(4-phenoxyphenyl)methanol | C13 H12 O2 | 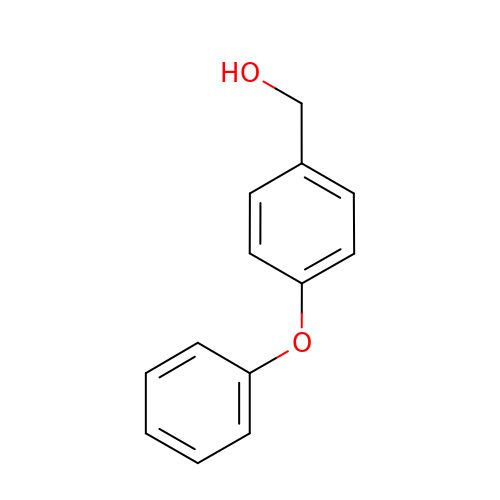FEOMFFKZOZMBKD-UHFFFAOYSA-N> MGKEALLNLYRIEYRPKDTTFTVFKPTHEIQKEKLNKVRWRVFLQTGLPTFRREDEFWCAGKVEKDTLYLTLSNGEIVELKRVGEEEFRGFQNERECQELFRDFLTKTKVKDKFISDFYKKFRDKITVQGKNRKIALIPEVNEKVLKSEEGYFLLHLDLKFRIQPFETLQTLLERNDFNPKRIRVKPIGIDFVGRVQDVFKAKEKGEEFFRLCMERSTHKSSKKAWEELLKNRELREKAFLVVLEKGYTYPATILKPVLTYENLEDEERNEVADIVRMEPGKRLNLIRYILRR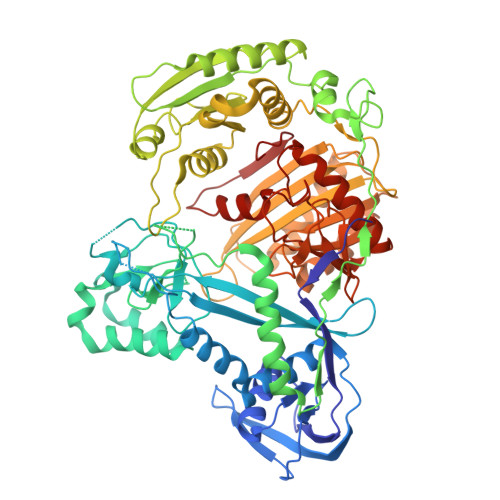YVKALRDYGWYISPEEERAKGKLNFKDTVLDAKGKNTKVITNLRKFLELCRPFVKKDVLSVEIISVSVYKKLEWRKEEFLKELINFLKNKGIKLKIKGKSLILAQTREEAKEKLIPVINKIKDVDLVIVFLEEYPKVDPYKSFLLYDFVKRELLKKMIPSQVILNRTLKNENLKFVLLNVAEQVLAKTGNIPYKLKEIEGKVDAFVGIDISRITRDGKTVNAVAFTKIFNSKGELVRYYLTSYPAFGEKLTEKAIGDVFSLLEKLGFKKGSKIVVHRDGRLYRDEVAAFKKYGELYGYSLELLEIIKRNNPRFFSNEKFIKGYFYKLSEDSVILATYNQVYEGTHQPIKVRKVYGELPVEVLCSQILSLTLMNYSSFQPIKLPATVHYSDKITKLMLRGIEPIKKEGDIMYWL>[4x]LPNITILATGGTIAGGGDSATKSNYTAGKVGVENLVNAVPQLKDIANVKGEQVVNIGSQDMNDNVWLTLAKKINTDCDKTDGFVITHGTDTMEETAYFLDLTVKCDKPVVMVGAMRPSTSMSADGPFNLYNAVVTAADKASANRGVLVVMNDTVLDGRDVTKTNTTDVATFKSVNYGPLGYIHNGKIDYQRTPARKHTSDTPFDVSKLNELPKVGIVYNYANASDLPAKALVDAGYDG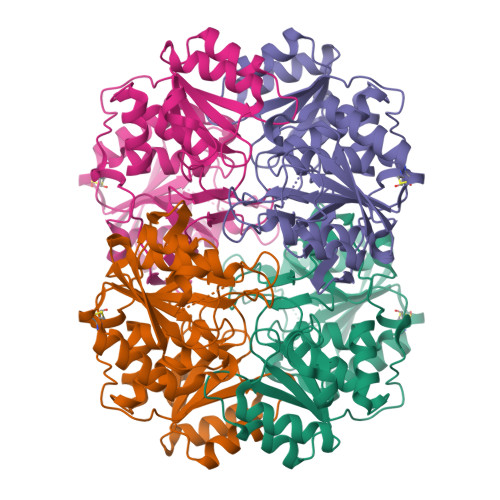IVSAGVGNGNLYKSVFDTLATAAKNGTAVVRSSRVPTGATTQDAEVDDAKYGFVASGTLNPQKARVLLQLALTQTKDPQQIQQIFNQY> GIQPVISAQEQETQIVLYGKLVEARQKHANKMDVPPAILATNKILVDMAKMRPTT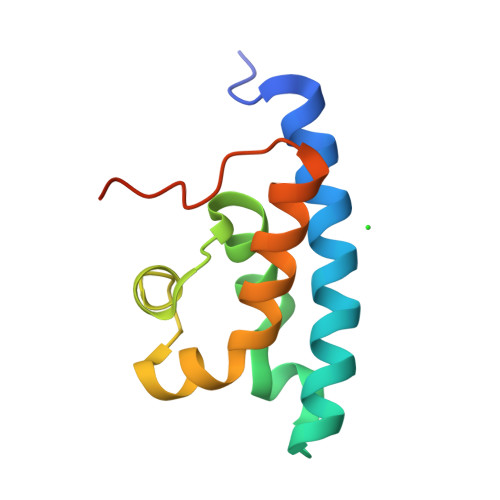VENVKRIDGVSEGKAAMLAPLLEVIKHFCQTNSVQTDLFSSTKPQEEQ>[8x]HHHHHHGSMTIKPLRKAVFPVAGLGTRFLPATKAMPKEMLPVVDRPLIQYAVDEAVEAGIEQMIFVTGRGKSALEDHFDIAYELEATMAARGKSLDVLDGTRLK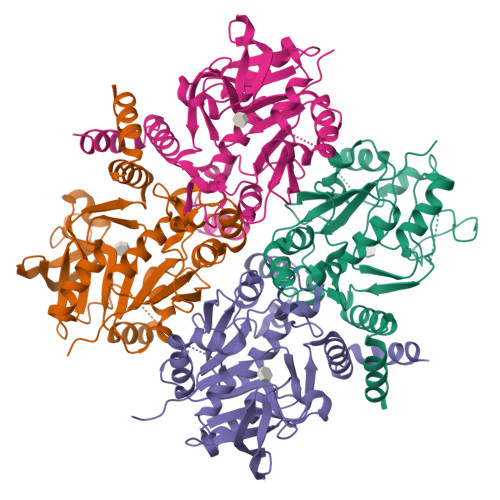PGNIAYVRQQEPMGLGHAVWCARDIVGDEPFAVLLPDDFMFGQPGCLKQMVDAYNKVGGNLICAEEVPDDQTHRYGIITPGTQDGVLTEVKGLVEKPAPGTAPSNLSVIGRYILQPEVMRILENQGKGAGGEIQLTDAMQRMIGDQPFHGVTFQGTRYDCGDKAGFIQANLAVALSRPDLEPAVRAFAVKALG> SNALQHTTIGDVLREHRRSHPGRTALVDGPVRLTWPELDDRVNRLAGSLAASGIGRGDRIMWLGQNSFRVYELIAAAGKLGAMVCVGYWRWAPPEMEFALRDFDPHLVVWQHQEIHETVARTREALGSDDTARWLRHDSAPQDPDGYEAFLAAGGLADPDLDIDPDSPVLVLYTAAMSGRQCGSLLSHTNLIAMATAAAWLGDIDHTTAFLNSGPMFHIGNHQFWGMPTLLMAGKNVIVRRV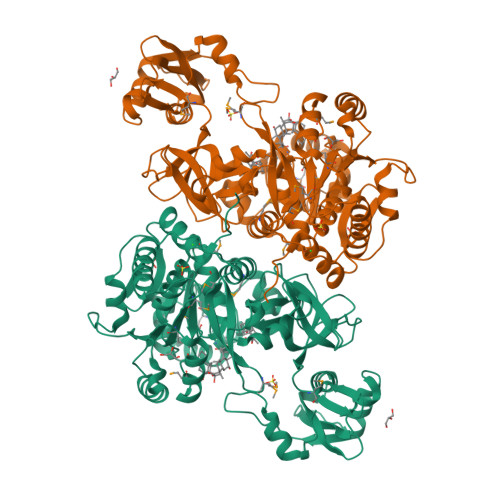VAEEVRDLLVAEECTHAFLMPPTVAEIVRLNRDTGHDLSRLRATVAPHLWEGMATTDTSRFTRSGAAAGRGYGQTELSGFAVTAAYGGPAAGNAGRPGPGLTVRVLDTAGRECAVGEAGEICARGTVVHRGYWNRDEVNAHRFRSGWWHTTDLGRREPDGSLTFLGTTTRMLKSAAENIFPAEVENCIEQHPAVREAAVIGVPNTRWAQDVKAVVVLEPDAGVSEQEIIDHCRPRIASYKKPKSVAFAAALPRTVSGARDYDALDKEYGGGGYPGAATLGPGR> MGSSHHHHHHSQDPKATWDIFCSVVDNYGDIGVTWRLARQLVAEHGLAVRLWVDDLNAFTPMCPGADATAAQQWQHGVDVRHWPAAWLPVAPADVVIGAFACQLPAAYVEAMRARPQPP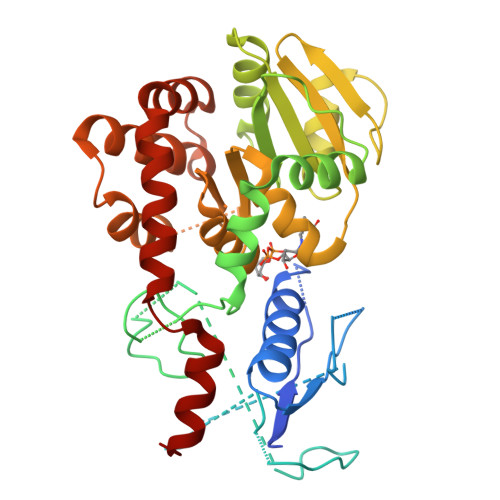LWLNLEYLSAEDWVEGCHGLPSPQPNGLRKVFFFPGFTDKTGGLLREGSLLARRDGFQQSAEARRAFLQGLGVDLVPGALLISLFAYENPQLGNWLDALATADQPCHLLVPQGRVVAGLSQWLGEGPLHVGDVRTRGALTVQVLPFVSQDDFDRLLWSCDFNAVRGEDSFVRAQWAGQPMLWHIYVQDENAHWEKLEAFLAHYRCGLSDDADAALLGLWRAWNMDFDMGQAWRAARQHWPELQQHARLWGARQAAQPDLATALVHFYRNSL>SMGFWEASSRGGGAFSGGEDASEGGAEEGAGGAGGSAGAGEGGVITALTPMTIPDVFPHLPLIAITRNPVFPRFIKIIEVKNKKLVELLRRKVRLAQPYVGVFLKRDDSNESDVVESLDEIYHTGTFAQIHEMQDLGDKLRMIVMGHRRVHISRQLEVEPEEPEAENKHKPRRKSKRGKKEAEDELSARHPAELAMEPTPELPAEVLMVEVENVVHEDFQVTEEVKALTAEIVKTIRDIIALNPLYRESVLQMMQAGQRVVDNPIYLSDMGAALTGAESHELQDVLEETNIPKRLYKALSLLKKEFELSKLQQRLGREVEEKIKQTHRKYLLQEQLKIIKKELGLEKDDKDAIEEKFRERLKELVVPKHVMDVVDEELSKLGLLDNHSSEFNVTRNYLDWLTSIPWGKYSNENLDLARAQAVLEEDHYGMEDVKKRILEFIAVSQLRGSTQGKILCFYGPPGVGKTSIARSIARALNREYFRFSVGGMTDVAEIKGHRWTYVGAMPGKIIQCLKKTKTENPLILIDEVDMIGRGYQGDPSSALLELLDPEQNANFLDHYLDVPVDLSKVLFICTANVTDTIPEPLRDRMEMINVSGYVAQEKLAIAERYLVPQARALCGLDESKAKLSSDVLTLLIKQYCRESGVRNLQKQVEKVLRKSAYKIVSGEAESVEVTPENLQDFVGKPVFTVERMYDVTPPGVVMGLAWTAMGGSTLFVETSLRRPQDKDAKGDKDGSLEVTGQLGEVMKESARIAYTFARAFLMQHAPANDYLVTSHIHLHVPEGATPKDGPSAGCTIVTALLSLAMGRPVRQNLAMTGEVSLTGKILPVGGIKEKTIAAKRAGVTCIVLPAENKKDFYDLAAFITEGLEVHFVEHYREIFDIAFPD[6x]

The hexameric, barrel-forming, AAA+ protease Lon is critical for maintaining mitochondrial matrix protein homeostasis. A human Lon monomer contains a mitochondrial targeting sequence, a Lon-associated N-terminal (LAN) domain, an α-helical neck region, an AAA+ domain, and a protease domain (PD) in a single chain. The LAN domains specifically recognize and capture fully or partially unfolded substrates, which are then threaded towards the barrel chamber for degradation using the chemical energy from ATP hydrolysis. We determined high-resolution structures of substrate-engaged, substrate-trapped, and substrate-free forms of the human mitochondrial Lon protease.

To gain further insight into the regulatory mechanisms of Lon protease activity we determined the cryo-EM structure of a substrate-free form of Lon (Lon^Apo^). We employed a fortuitously stable, catalytically inactive Lon mutant (containing the mutations G106P, R563W, and K594M), which also displays no proteolytic activity and limited ATPase activity. The Lon^Apo^ has a right-handed helical arrangement with a rise of approximately 8 Å ([Fig fig4], Fig. S4C) and all protomers are ADP-bound. The catalytic S855 is in an α-helix preceded by a loop (residues 844– 852, [Fig fig4]) that functions as a gate controlling the accessibility to the catalytic site. In Lon^Apo^, this gate loop is in a closed conformation ([Fig fig4]). The C-terminal part of the loop forms a 3_10_ helical turn, thereby extending the S855-containing α-helix. The turn is stabilized by a salt bridge between K851 and D643 in the α-subdomain. The 3_10_ helical turn positions the key residue D852 to form a salt-bridge with the catalytic K898 ([Fig fig4] and Fig. S6B) and hinders the proteolytic activity.The Marasmius oreades agglutinin (MOA) is the holotype of an emerging family of fungal chimerolectins and an active Ca2+/Mn2+-dependent protease, which exhibits a unique papain-like fold with special active site features. While acting as a dimerization domain, the papain-like domain of MOA retains the characteristic L-/R-domain partition of PLCPs. As additional feature, the MOA dimer carries two binuclear metal-binding clusters, symmetrically placed at the dimerization interface (Grahn et al., 2009). MOA requires the presence of calcium or manganese (II) to switch from the inactive form to an active protease (Cordara et al., 2011, Wohlschlager et al., 2011).

In an effort to validate our substrate binding model, we co-crystallized the enzymatically inactive MOA variants C215A and C215A/H257A with two synthetic heptapeptides mimicking proteolytic substrates. The designed peptides have the sequence PVxRAHS (with x = P or V). Unexpectedly, co-crystallization of catalytically inactive MOA variants with different substrate mimics resulted in complexes of the enzyme with cleaved peptides. The observed cleavage products correspond to the N-terminal proteolytic fragments, binding to the MOA active site in the standard backbone orientation expected for PLCP substrates. The synthetic peptides are anchored to the active site through three main contact points: the oxyanion hole, defined by Trp208 and the backbone NH group of Ala215, the ‘site B’ Ca2+ ion and a backbone–backbone interaction with Ala256. The presence of an arginine residue at the P1 position unambiguously maps the S1 subsite to the carboxylate group of L-domain Glu210, which forms a side-on bidentate salt bridge with the Arg guanidinium group. The P2 moiety binds to the S2 specificity pocket lined by residues Leu247, Ala258 and Leu182# (with ‘#’ identifying a residue provided by the other subunit). The peptide complex structures show well-defined electron density accounting for the N-terminal fragment of the substrate mimics after proteolytic cleavage, representing one of few examples of PLCP structures in complex with a proteolysis product. Substrate activation by the oxyanion hole combined with water-catalyzed hydrolysis is a known source of residual activity in proteases (Carter and Wells, 1988, Corey and Craik, 1992, Krishnan et al., 2000) and has also been observed in PLCPs. Coupled to the long time needed to grow the crystals (2–3 weeks), this could explain the presence of a cleaved peptide rather than the full substrate.

> MSLRRGIYHIENAGVPSAIDLKDGSSSDGTPIVGWQFTPDTINWHQLWLAEPIPNVADTFTLCNLFSGTYMDLYNGSSEAGTAVNGWQGTAFTTNPHQLWTIKKSSDGTSYKIQNYGSKTFVDLVNGDSSDGAKIAGWTGTWDEGNPHQKWYFNRMSVSSAEAQAAIARNPHIHGTYRGYILDGEYLVLPNATFTQIWKDSGLPGSKWREQIYDCDDFAIAMKAAVGKWGADSWKANGFAIFCGVMLGVNKAGDAAAAYNFTLTKDHADIVFFEPQNGGYLNDIGYDSYMAFY;> PVPRAHS The semaphorins are the largest family of evolutionarily conserved axon guidance cues. The semaphorins signal through their main receptors, plexins, which are single-spanning transmembrane proteins expressed in a variety of cell types, including neurons, cancer cells or endothelial cells. We determined crystal structures of Drosophila Sema1a1–2, Sema1b1–2, Sema2a1–3 and Sema2b1–3 to a 3.6-, 2.8-, 2.1- and 2.5 -Å resolution, respectively. All structures contain the sema domain composed of a seven-bladed β-propeller fold, which is followed by a PSI domain.

In the crystal, Sema1a1–2, Sema2a1–3 and Sema2b1–3 form a disulfide-linked dimer, while Sema1b1–2 is a monomer and the lattice packing provides no evidence for Sema1b1–2 dimerization within the crystal. In Sema1b, the equivalent cysteine residue at position 254 is naturally substituted by a phenylalanine, and thus Sema1b fails to form the interchain disulfide bond as compared with Sema1a, Sema2a and Sema2b. When we mutated the phenylalanine 254 in Sema1becto to cysteine, we observed a mixture of a monomer and a disulfide-linked dimer similar to that of Sema1aecto. The low propensity to non-covalently dimerize and the natural substitution of cysteine 254 to phenylalanine together contribute to the monomeric state of Sema1becto. We further found that Sema1b lacks this bond and our crystal structure determination and biophysical data in solution all show Sema1becto to be in a monomeric state due to the C254F substitution. The monomeric structure of Sema1becto we report here raises the intriguing possibility that semaphorin function may not be restricted to dimers, but also monomers could contribute to the complexity of biology mediated by the semaphorin family. In class 1 semaphorins, two distinct loops with no obvious structural and functional role are substantially extended from the bottom face of the β-propeller, β5A–β5B and β7A–β7B in Sema1a, and β2C–β2D and β6C–β6D Sema1b. The latter loops in Sema1b also showed a higher level of fluctuations relative to the rest of protein in the molecular dynamics simulations. Intriguingly, we found that the cytoplasmic domain of Sema1b lacks the sequence previously determined to be crucial for reverse signalling of Sema1a22,31, and therefore, Sema1b might be incapable of mediating reverse signalling.

> ETGDVKPDLQTKQDKVLAHFIGNSTDYFKILDHNDEFVLVGAKDVIYNVSLNGLKEIARLEWHSTDADRELCALKGKHEWDCHNYLRVYALRPNGEVLLCGTNSYKPRCRHYTPVEVSSEEAGSAGHAHAMRYEVSRDVEAQGLCPYSPAHNSTYAFADGHLYSATVADFSGGDPLIYRENLRTEQYDLKQLNQPDFVGAIERNGYVLFFFRELSMEVMNFGKAVYSRVARVCKNDRGGPYSHGKSWTSFLKARLNCSVPGEFPFYFDEIQAISPIVESGSKSLIYAVFTTSVNAIPGSAVCAFNVDDILAAFDGEFKSQKDSQSHWLPVEREQVPKPRPGQCVEDSRTLTSIAVNFIKNHPLMEEAVPAVHGRPLLTKVNLHHRLTAIAVHPQVKSLSGAYYDVIYSGTDDGKVTKFINILSTHPNSTVDRLKTVVISEMQVLPLGTPIRELVISTSKNSLVVVSDGSLVSVPLHHCSHIVDCLGCLSLQDPICAWDLQTHECKNLATSQHKFGTKTYLQSLNSTKKAAALLCPHIPRDAPGAETVSFVTMAPPPTEEQKLLYSNVGSGTKHHHHHH>[2x]GSTLTYPFHDWSQELSPRYAQLRASDAPVCPVVSEGTGDPLWLVTRYATAVKLLEDSRFSSEAAQASGAPRQEPVELRAPGTRGDAIAMLREAGLRSVLADGLGPRAVRRHQGWINDLAETLMSELASREGTFDLAADFVEPLSSALVSRTLLGELSADERDLLAHCADTGLRFCGVTHEEQVHAFTQMHEFFLEHARRLAGTPGEHLLKLIAEAPVDQGPLSDEALAEAGSLLVVAGFPTSSGFLCGALLTLLRHPDAVQELHAHPERVPSAVEELLRYTPLSTGSVKRMATEDLEIDGVRIKAGEVVMVSLEAVNHDPDAFEDPDVFRPGREGPMHFGFGRGRHFCPGNRLARCVIEATVRAVARRPGLRLAVAPEEISWHEGLFFRRPRAIPATW

Further, the in vitro assay confirmed that NasF5053 could produce NAS-C (47.4%), Asp-A (44.4%), as well as a minor product NAS-B (8.2%) (trace I). NasF5053 adopts the prism-like fold characteristic for P450s, consisting of a large domain of 10-helices (C-L) and a small domain of four α-helices (A, B, B’, and K’) and three β-sheets (strands β1-1 to 4, β2-1 to 2, and β3-1 to 2). Our systematic mutagenesis studies on the promiscuous NasF5053 and the versatile NascB identified four key resides, Q65, A86, S284, and V288, which play critical roles in controlling product regio-configurations and stereo-configurations. To obtain insights into the structural basis for regio-specificity, stereo-specificity, and chemical versatility, we further determined high-resolution crystal structures of wild-type NasF5053 in its substrate-free and substrate-bound form, and of two NasF5053 mutants (Q65I-A86G and S284A-V288A) in their substrate-bound forms.

Comparison between the substrate-free and substrate-bound NasF5053 structures reveals binding of substrates only invokes minimal conformational changes, with a root-mean-square deviation (RMSD) of 0.362 Å (for 388 Cα atoms) between the two forms. Instead, substrate binding is associated with rearrangements of some of the residues lining the substrate-binding cavity. Upon substrate binding, the side-chains of both D85 and E73 rotate along the Cα-Cβ axis away from the binding site, to accommodate the substrates. Q65 undergoes a 2.0 Å shift (measured on the Cδ atom) toward the binding site, to interact with one of the substrate molecules (cWL-PL-U; see below). Notably, Q65, D85, and E73 all reside in the long αB’-αC loop.> MWSHPQFEKASTGREILEKLERREFTREVLKEALSINDRGFNEALFKLADEIRRKYVGDEVHIRAIIEFSNVCRKNCLYCGLRRDNKNLKRYRMTPEEIVERARLAVQFGAKTIVLQSGEDPYYMPDVISDIVKEIKKMGVAVTLSLGEWPREYYEKWKEAGADRYLLRHETAN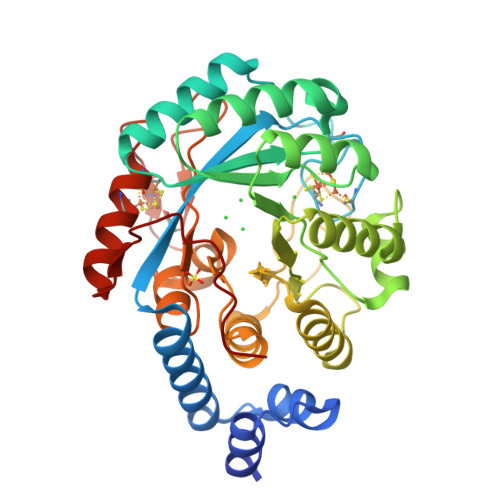PVLHRKLRPDTSFENRLNCLLTLKELGYETGAGSMVGLPGQTIDDLVDDLLFLKEHDFDMVGIGPFIPHPDTPLANEKKGDFTLTLKMVALTRILLPDSNIPATTAMGTIVPGGREITLRCGANVIMPNWTPSPYRQLYQLYPGKICVFEKDTACIPCVMKMIELLGRKPGRDWGGRKRVFETV> MLDPNLLRTEPDAVAEKLARRGFKLDVDKLRALEERRKVLQVQTENLQAERNSRSKSIGQAKARGEDIEPLRLEVNKLGEQLDAAKSELETLLAEIR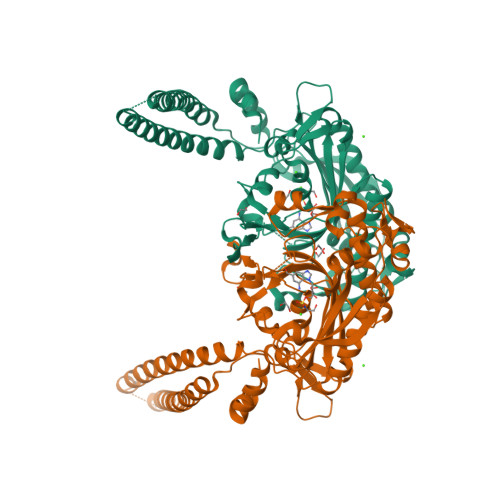DIALAIPNIPHDDVPVGRDENDNVEVSRWGTPRQFDFEVRDHVTLGEMHGGLDFAAAVKLTGSRFVVMKGQLARLHRALAQFMLDLHTEQHGYSENYVPYLVNQDTLYGTGQLPKFAGDLFHTRPLEEEADSSNYALIPTAEVPLTNLVRDEIIDEDDLPIKMTAHTPCFRSEAGSYGRDTRGLIRMHQFDKVEMVQIVRPEDSMAALEEMTGHAEKVLQLLGLPYRKVALCTGDMGFSACKTYDLEVWVPAQNTYREISSCSNVWDFQARRMQARCRSKSDKKTRLVHTLNGSGLAVGRTLVALMENYQQADGRIEIPEVLRPYMRGLEYIG>[4x]MNKVYLANAFSINMLTKFPTKVVIDKIDRLEFCENIDNEDIINSIGHDS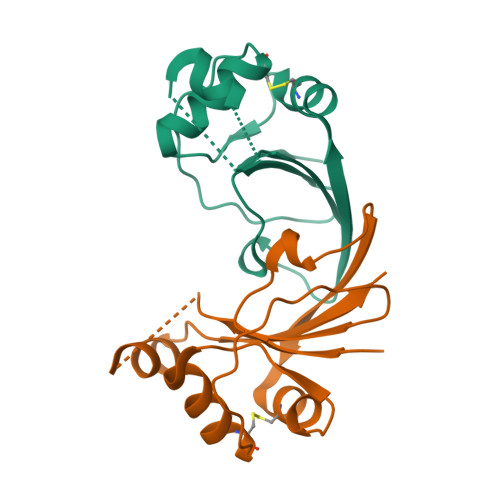TIQLINSLCGTTFQKNRVEIKLEKEDKLYVVQISQRLEEGKILTLEEILKLYESGKVQFFEIIVD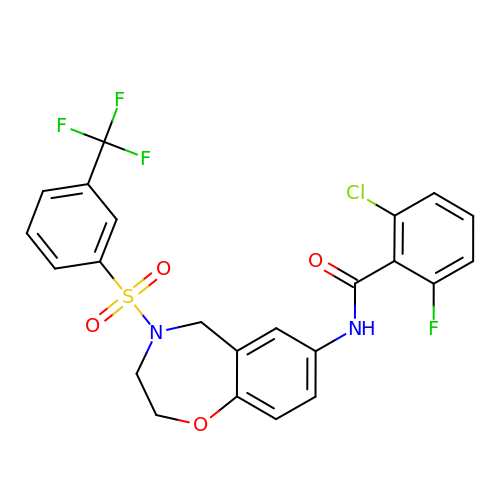2-CHLORO-6-FLUORO-N-[4-[3-(TRIFLUOROMETHYL)PHENYL]SULFONYL-3,5-DIHYDRO-2H-1,4-BENZOXAZEPIN-7-YL]BENZAMIDE | C23 H17 Cl F4 N2 O4 S | BCCOZQIHZZQJIS-UHFFFAOYSA-N>[2x]MSQTHKHAIPANIADRCLINPEQYETKYKQSINDPDTFWGEQGKILDWITPYQKVKNTSFAPGNVSIKWYEDGTLNLAANCLDRHLQENGDRTAIIWEGDDTSQSKHISYRELHRDVCRFANTLLDLGIKKGDVVAIYMPMVPEAAVAMLACARIGAVHSVIFGGFSPEAVAGRIIDSSSRLVITADEGVRAGRSIPLKKNVDDALKNPNVTSVEHVIVLKRTGSDIDWQEGRDLWWRDLIEKASPEHQPEAMNAEDPLFILYTSGSTGKPKGVLHTTGGYLVYAATTFKYVFDYHPGDIYWCTADVGWVTGHSYLLYGPLACGATTLMFEGVPNWPTPARMCQVVDKHQVNILYTAPTAIRALMAEGDKAIEGTDRS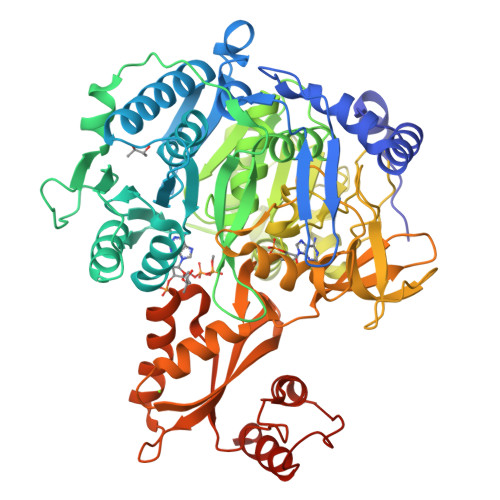SLRILGSVGEPINPEAWEWYWKKIGKEKCPVVDTWWQTETGGFMITPLPGAIELKAGSATRPFFGVQPALVDNEGHPQEGATEGNLVITDSWPGQARTLFGDHERFEQTYFSTFKNMYFSGDGARRDEDGYYWITGRVDDVLNVSGHRLGTAEIESALVAHPKIAEAAVVGIPHAIKGQAIYAYVTLNHGEEPSPELYAEVRNWVRKEIGPLATPDVLHWTDSLPKTRSGKIMRRILRKIAAGDTSNLGDTSTLADPGVVEKLLEEKQAIAMPSLEHHHHHH> MMIRGIRGATTVERDTEEEILQKTKQLLEKIIEENHTKPEDVVQMLLSATPDLHAVFPAKA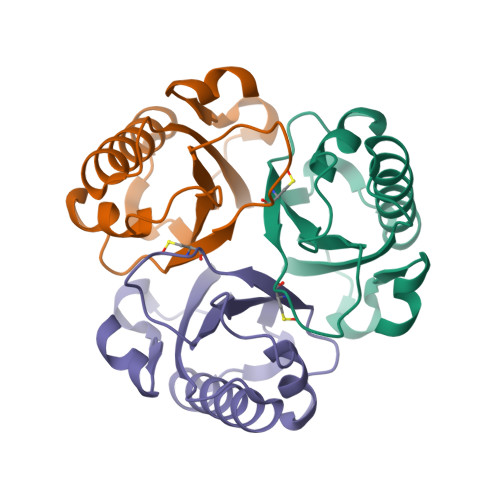VRELSGWQYVPVTCMQEMDVTGGLKKSIKVMMTVQTDVPQDQIRHVYLEKAVVLRPDLSLTKNTEL Tyrosinases (TYRs, EC 1.14.18.1 and EC 1.10.3.1) and catechol oxidases (COs, EC 1.10.3.1) are type III copper‐containing metalloenzymes that constitute the class of polyphenol oxidases (PPOs). More specifically, plant PPOs are expressed as pro‐enzymes (55–65 kDa) consisting of an enzymatically active (40–45 kDa) and a C‐terminal domain (15–19 kDa). The C‐terminal domain plays a significant role in the regulation of the enzyme activity inside the cell by shielding the catalytic pocket of the active centre, and in addition it provides an indispensable motif for the accurate folding of the active domain. Herein, we investigated the activation of PPO1 from Malus domestica (MdPPO1) and present a novel activation mode for plant PPOs driven by self‐cleavage, which is independent of external proteases or any other harsh conditions (e.g., SDS).

To corroborate this result, an orthogonal experiment was performed, where the sole C‐terminal domain was recombinantly overexpressed (Csole‐domain) and crystallized. In summary, we have recombinantly produced and successfully crystallized the pro‐form of MdPPO1 and two versions of its C‐terminal domain, one obtained after self‐cleavage (Ccleaved) and the other one as an independently expressed domain (Csole). Structural analysis of the separated C‐terminal domains, Ccleaved and Csole, revealed a metal‐binding site. The bound metal was identified as Ca2+ based on the composition of the used expression media and buffers, the interacting amino acids, the binding geometry, and the presence of anomalous signal. This binding site is absent in the C‐terminal domain still attached to the pro‐enzyme. Moreover, pro‐MdPPO1 was incubated with different amounts of Csole‐domain to investigate whether the C‐terminal domain plays a role in the self‐cleavage process. The results clearly demonstrate that the addition of (external) Csole‐terminal domain significantly increases the self‐cleavage rate as with increasing concentration of external Csole‐domain, the pro‐enzyme is cleaved into its active and C‐terminal domain faster.

> GPAAVASSSKVVAGTEFPISLGSKISTVVKRPKQKKRSKKAKEDEEEILVIEGIEFDRDVAVKFDVYVNDVDDLPSGPDKTEFAGSFVSVPHSHKHKKKMNTILRLGLTDLLEEIEAEDDDSVVVTLVPKFGAVKIGGIKIEFAS>MKLPLLLALLFGAVSALHLRSETSTFETPLGAKTLPEDEETPEQEMEETPCRELEEEEEWGSGSEDASKKDGAVESISVPDMVDKNLTCPEEEDTVKVVGIPGCQTCRYLLVRSLQTFSQAWFTCRRCYRGNLVSIHNFNINYRIQCSVSALNQGQVWIGGRITGSGRCRRFQWVDGSRWNFAYWAAHQPWSRGGHCVALCTRGGHWRRAHCLRRLPFICSY[2x];>[2x]MRLWSWVLHLGLLSAALGCGLAERPRRARRDPRAGRPPRPAAGPATCATRAARGRRASPPPPPPPGGAWEAVRVPRRRQQREARGATEEPSPPSRALYFSGRGEQLRLRADLELPRDAFTLQVWLRAEGGQRSPAVITGLYDKCSYISRDRGWVVGIHTISDQDNKDPRYFFSLKTDRARQVTTINAHRSYLPGQWVYLAATYDGQFMKLYVNGAQVATSGEQVGGIFSPLTQKCKVLMLGGSALNHNYRGYIEHFSLWKVARTQREILSDMETHGAHTALPQLLLQENWDNVKHAWSPMKDGSSPKVEFSNAHGFLLDTSLEPPLCGQTLCDNTEVIASYNQLSSFRQPKVVRYRVVNLYEDDHKNPTVTREQVDFQHHQLAEAFKQYNISWELDVLEVSNSSLRRRLILANCDISKIGDENCDPECNHTLTGHDGGDCRHLRHPAFVKKQHNGVCDMDCNYERFNFDGGECCDPEITNVTQTCFDPDSPHRAYLDVNELKNILKLDGSTHLNIFFAKSSEEELAGVATWPWDKEALMHLGGIVLNPSFYGMPGHTHTMIHEIGHSLGLYHVFRGISEIQSCSDPCMETEPSFETGDLCNDTNPAPKHKSCGDPGPGNDTCGFHSFFNTPYNNFMSYADDDCTDSFTPNQVARMHCYLDLVYQGWQPSRKPAPVALAPQVLGHTTDSVTLEWFPPIDGHFFERELGSACHLCLEGRILVQYASNASSPMPCSPSGHWSPREAEGHPDVEQPCKSSVRTWSPNSAVNPHTVPPACPEPQGCYLELEFLYPLVPESLTIWVTFVSTDWDSSGAVNDIKLLAVSGKNISLGPQNVFCDVPLTIRLWDVGEEVYGIQIYTLDEHLEIDAAMLTSTADTPLCLQCKPLKYKVVRDPPLQMDVASILHLNRKFVDMDLNLGSVYQYWVITISGTEESEPSPAVTYIHGSGYCGDGIIQKDQGEQCDDMNKINGDGCSLFCRQEVSFNCIDEPSRCYFHDGDGVCEEFEQKTSIKDCGVYTPQGFLDQWASNASVSHQDQQCPGWVIIGQPAASQVCRTKVIDLSEGISQHAWYPCTISYPYSQLAQTTFWLRAYFSQPMVAAAVIVHLVTDGTYYGDQKQETISVQLLDTKDQSHDLGLHVLSCRNNPLIIPVVHDLSQPFYHSQAVRVSFSSPLVAISGVALRSFDNFDPVTLSSCQRGETYSPAEQSCVHFACEKTDCPELAVENASLNCSSSDRYHGAQCTVSCRTGYVLQIRRDDELIKSQTGPSVTVTCTEGKWNKQVACEPV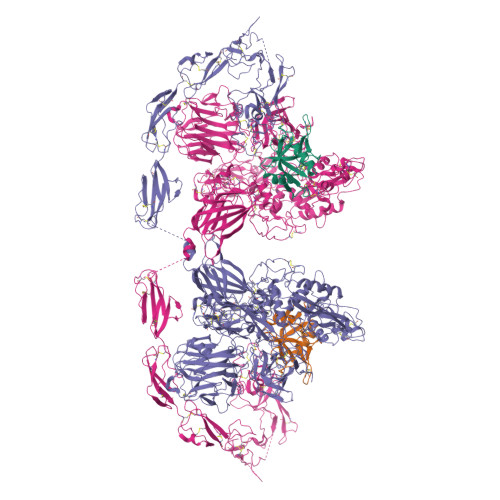DCSIPDHHQVYAASFSCPEGTTFGSQCSFQCRHPAQLKGNNSLLTCMEDGLWSFPEALCELMCLAPPPVPNADLQTARCRENKHKVGSFCKYKCKPGYHVPGSSRKSKKRAFKTQCTQDGSWQEGACVPVTCDPPPPKFHGLYQCTNGFQFNSECRIKCEDSDASQGLGSNVIHCRKDGTWNGSFHVCQEMQGQCSVPNELNSNLKLQCPDGYAIGSECATSCLDHNSESIILPMNVTVRDIPHWLNPTRVERVVCTAGLKWYPHPALIHCVKGCEPFMGDNYCDAINNRAFCNYDGGDCCTSTVKTKKVTPFPMSCDLQGDCACRDPQAQEHSRKDLRGYSHG>[2x]GMTSRSPFESFVWQSEIFNCQSNDIDAFYAQLAEEVNRLGLKKNTLGSVDSFAINLYQSASQRSDLPSLLISSGFHGEEAAGPWGMLHFLRGLQPALFERVNLSLLPLVNPTGFKAGHRFNRFGENPNRGFTLE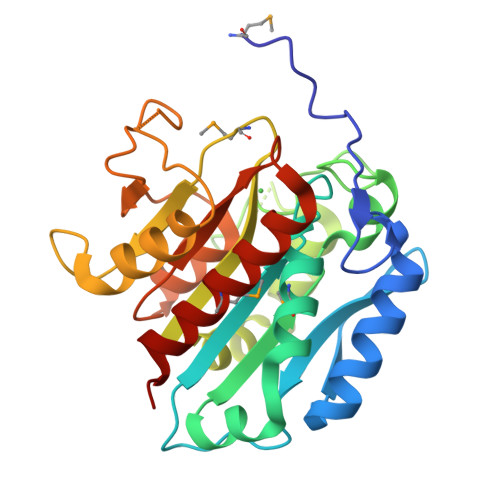NGKPTPNEHTSLEGKLLLEHAQLLCAASRDGILTCHEDVLMNETYVYSFEPTQTPGRFSLGLRDALGQYFKLAKDGFIDECPVTDGVIFNHFDTSFEAFLVRSGAKLAACSETPGQEDFDRRVQANSAAMGQFIAHCAPIL>MALNKNMFSSLFLGYLLVYATTVQSSIHYDSLSKVGVIKGLTYNYKIKGSPSTKLMVVKLIPNIDSVKNCTQKQYDEYKNLVRKALEPVKMAIDTMLNNVKSGNNKYRFAGAIMAGVALGVATAATVTAGIALHRSNENAQAIANMKSAIQNTNEAVKQLQLANKQTLAVIDTIRGEINNNIIPVINQLSCDTIGLSVGIRLTQYYSEIITAFGPALQNPVNTRITIQAISSVFNGNFDELLKIMGYTSGDLYEILHSELIRGNIIDVDVDAGYIALEIEFPNLTLVPNAVVQELMPISYNIDGDEWVTLVPRFVLTRTTLLSNIDTSRCTITDSSVICDNDYALPMSHELIGCLQGDTSKCAREKVVSSYVPKFALSDGLVYANCLNTICRCMDTDTPISQSLGATVSLLDNKRCSVYQVG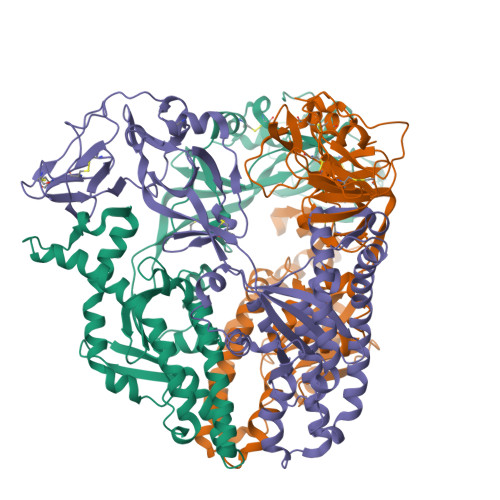DVLISVGSYLGDGEYNADNVELGPPIVIDKIDIGNQLAGINQTLQEAEDYIEKSEEFLKG[3x]>GGVFPNVTNINSDKLLGGLLASGFDEDSCLSRYQSVHYRKPSPYKPSSYLISKLRNYEKLHKRCGPGTESYKKALKQLDQEHIDGDGECKYVVWISFSGLGNRILSLASVFLYALLTDRVLLVDRGKDMDDLFCEPFLGMSWLLPLDFPMTDQFDGLNQESSRCYGYMVKNQVIDTEGTLSHLYLHLVHDYGDHDKMFFCEGDQTFIGKVPWLIVKTDNYFVPSLWLIPGFDDELNKLFPQKATVFHHLGRYLFHPTNQVWGLVTRYYEAYLSHADEKIGIQVRVFDEDPGPFQHVMDQISSCTQKEKLLPEVDTLVERSRHVNTPKHKAVLVTSLNAGYAENLKSMYWEYPTSTGEIIGVHQPSQEGYQQTEKKMHNGKALAEMYLLSLTDNLVTSAWSTF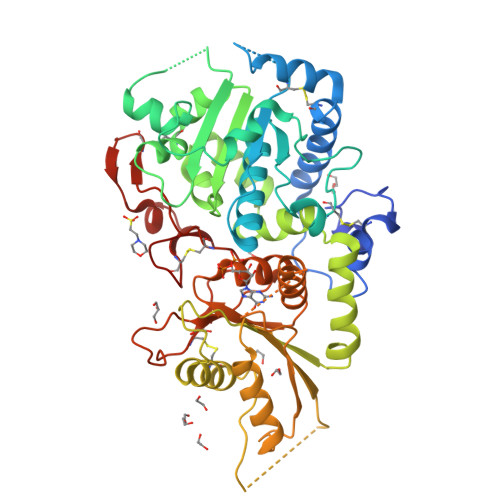GYVAQGLGGLKPWILYRPENRTTPDPSCGRAMSMEPCFHSPPFYDCKAKTGIDTGTLVPHVRHCEDISWGLKLV[2x]> MKVLYFAEIKDILQKAQEDIVLEQALTVQQFEDLLFERYPQIN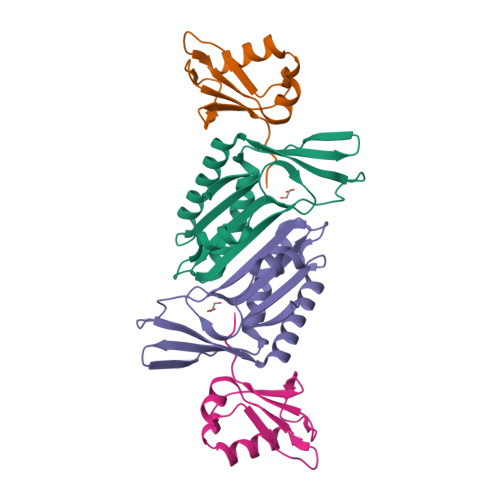NKKFQVAVNEEFVQKSDFIQPNDTVALIPPVSGG;> HMKQFEIVIEPIQTEQYREFTINEYQGAVVVFTGHVREWTKGVKTEYLEYEAYIPMAEKKLAQIGDEINEKWPGTITSIVHRIGPLQISDIAVLIAVSSPHRKDAYRANEYAIERIKEIVPIWKKEIWEDGSKWQGHQKGNYEEAKREE>[4x]MGSTPTDT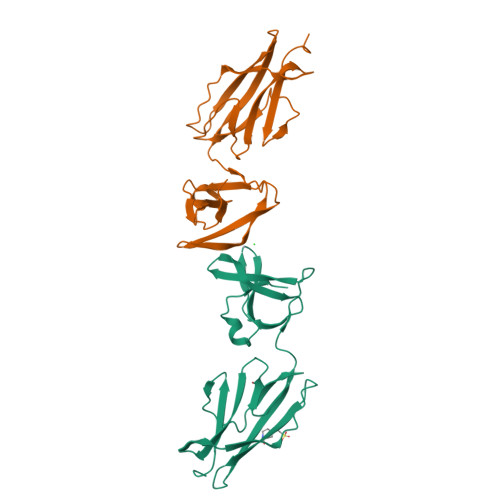TQNPQINWTKGGQAQSSSLNGQVFQVAVGSNFNPLNFTNSNGENIIVSAQQSKNNTTFASIEATSNPVNTSEAGRYYNVTLTATGNTGKKTTATYTVLITSSQKQTLYGNGESTISTYSIYGNNVLCNSTTFKDGDQVYVSDQTKTVGGVSYSQVSPKSKNDANSSNIWVKTSLEHHHHHH> SNAMGNSTPHSLHSDAICIGFGPAGIALACAFEDAREASQPLGDLSIGYLEAAPDTQWHRELLLAGTDINHHVFRDLVTPRNPRSRFSFAMYLKDQGRMFDFGLLGRPASRHEWSDYLGWVSRQVDGHTRFDTPVTEIDPVIRNGRLQE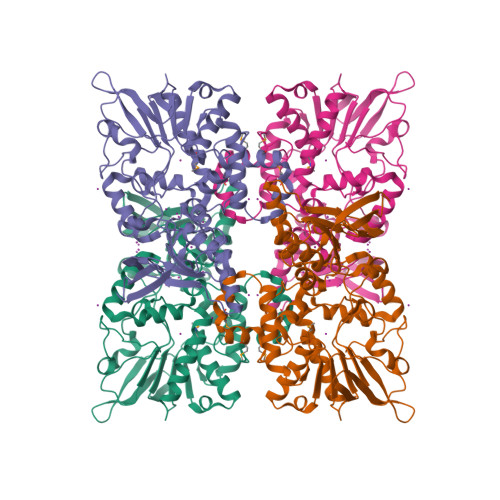VRVRTPQGSFATRNLVLSSGSAPRIPQAFEALLGPTLFHTSRFLTRLQAFGKQLPKRWLVLGSGQSASESVLELVSRDPAIEVHSVHRCAGFKLTQLGQFPNRVFAPDHVDYFHSLNPAARQRFLDWSRSTNYAGIDPDERQKLFSLIYEDSIAGRTRLHTYAYSVISAIEHTADGYRVELTDTFSQRTRVLEVDAVVLGTGYQQYLIPPLLSGLQPWLAADVDGGLLIDRDYRVATQGACDVNIWVNGLSERSHGISDSQSFSLMALRAGRIASALERAVEPATDAPLLAQWT> MAKQRVFIAGHRGMVGSAIRRQLEQRGDVELVLRTRDELNLLDSRAVHDFFASERIDQVYLAAAKVGGIVANNTYPADFIYQNMMIESNIIHAAHQNDVNKLLFLGSSCIYPKLAKQPMAESELLQGTLEPTNEPYAIAKIAGIKLCESYNRQYGR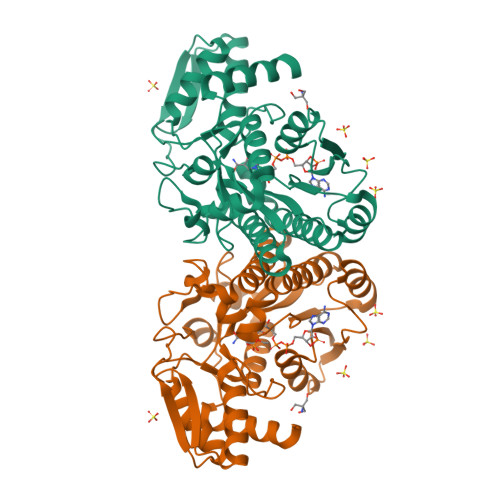DYRSVMPTNLYGPHDNFHPSNSHVIPALLRRFHEATAQKAPDVVVWGSGTPMREFLHVDDMAAASIHVMELAHEVWLENTQPMLSHINVGTGVDCTIRELAQTIAKVVGYKGRVVFDASKPDGTPRKLLDVTRLHQLGWYHEISLEAGLASTYQWFLENQDRFRG AaRSs catalyze the attachment of the correct amino acid to its cognate tRNA which then is used in protein synthesis on ribosomes. Phylogenetically phenylalanyl-tRNA synthetase (PheRS), belongs to the class II aaRSs, and it is a dimer of heterodimers (αβ)2, containing two α- (PheS) and two β- (PheT) subunits. Structural studies of PheRS have shown that the α subunit binds L-Phe and ATP and is responsible for esterification catalysis. At the same time, the β subunit is involved in the recognition of the cognate tRNA molecule and editing of mis-charged tRNA.

The protein-fragment interactions were analyzed using crystal structures for five of those fragments complexed with MtPheRS/tRNAPhe (DDD00107555 (D-555), DDD01008876 (D-876), DDD00805735 (D-735), DDD00079004 (D-004) and DDD00067116 (D-116)). All five fragments occupy the L-Phe site in the α subunit of the heterotetramer. The bicyclic quinoline, quinazoline and benzimidazole moieties of the fragments are completely enclosed in the L-Phe binding site. PIEDA showed that the phenyl ring or the bicyclic core of the fragments interact with residues αPhe255 and αPhe257 through hydrophobic interaction. Residues αThr258 and αAla305 make hydrophobic interactions with the phenyl core of the fragments D-116, D-004 and D-735. FMO analysis showed a strong hydrogen bond between the proton of NH2 moiety in D-004 and residue αGlu217. Hydrophobic interactions with αAla305 are retained in fragments D-735, D-004 and D-116. However, the auxiliary pocket in the structures of PheRS with bound fragments was completely unoccupied offering an opportunity for fragment growth by adding hydrophobic substituents to explore the auxiliary pocket of MtPheRS.

>[2x]ENLYFQSNAMLSPEALTTAVDAAQQAIALADTLDVLARVKTEHLGDRSPLALARQALAVLPKEQRAEAGKRVNAARNAAQRSYDERLATLRAERDAAVLVAEGIDVTLPSTRVPAGARHPIIMLAEHVADTFIAMGWELAEGPEVETEQFNFDALNFPADHPARGEQDTFYIAPEDSRQLLRTHTSPVQIRTLLARELPVYIISIGRTFRTDELDATHTPIFHQVEGLAVDRGLSMAHLRGTLDAFARAEFGPSARTRIRPHFFPFTEPSAEVDVWFANKIGGAAWVEWGGCGMVHPNVLRATGIDPDLYSGFAFGMGLERTLQFRNGIPDMRDMVEGDVRFSLPFGVGA;>[2x]QSNAMRLPYSWLREVVAVGASGWDVTPGELEQTLLRIGHEVEEVIPLGPVDGPVTVGRVADIEELTGYKKPIRACAVDIGDRQYREIICGATNFAVGDLVVVALPGATLPGGFTISARKAYGRNSDGMICSAAELNLGADHSGILVLPPGAAEPGADGAGVLGLDDVVFHLAITPDRGYCMSVRGLARELACAYDLDFVDPASNSRVPPLPIEGPAWPLTVQPETGVRRFALRPVIGIDPAAVSPWWLQRRLLLCGIRATCPAVDVTNYVMLELGHPMHAHDRNRISGTLGVRFARSGETAVTLDGIERKLDTADVLIVDDAATAAIGGVMGAASTEVRADSTDVLLEAAIWDPAAVSRTQRRLHLPSEAARRYERTVDPAISVAALDRCARLLADIAGGEVSPTLTDWRGDPPCDDWSPPPIRMGVDVPDRIAGVAYPQGTTARRLAQIGAVVTHDGDTLTVTPPSWRPDLRQPADLVEEVLRLEGLEVIPSVLPPAPAGRGLTAGQQRRRTIGRSLALSGYVEILPTPFLPAGVFDLWGLEADDSRRMTTRVLNPLEADRPQLATTLLPALLEALVRNVSRGLVDVALFAIAQVVQPTEQTRGVGLIPVDRRPTDDEIAMLDASLPRQPQHVAAVLAGLREPRGPWGPGRPVEAADAFEAVRIIARASRVDVTLRPAQYLPWHPGRCAQVFVGESSVGHAGQLHPAVIERSGLPKGTCAVELNLDAIPCSAPLPAPRVSPYPAVFQDVSLVVAADIPAQAVADAVRAGAGDLLEDIALFDVFTGPQIGEHRKSLTFALRFRAPDRTLTEDDASAARDAAVQSAAERVGAVLRG> MAQFYSAKRRTTTRQIITVSVNDLDSFGQGVARHNGKTLFIPGLLPQENAEVTVTEDKKQYARAKVVRRLSDSPERETPRCPHFGVCGGCQQQHASVDLQQRSKSAALARLMKHDVSEVIADVPWGYRRRARLSLNYLPKTQQLQMGFRKAGSSDIVDVKQCPILAPQLEALLPKVRACLGSLQAMRHLGHVELVQATSGTLMILRHTAPLSSADREKLERFSHSEGLDLYLAPDSEILETVSGEM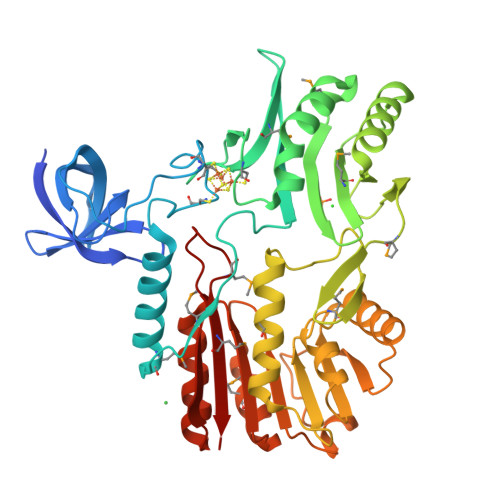PWYDSNGLRLTFSPRDFIQVNAGVNQKMVARALEWLDVQPEDRVLDLFCGMGNFTLPLATQAASVVGVEGVPALVEKGQQNARLNGLQNVTFYHENLEEDVTKQPWAKNGFDKVLLDPARAGAAGVMQQIIKLEPIRIVYVSCNPATLARDSEALLKAGYTIARLAMLDMFPHTGHLESMVLFSRVK>MGSSHHHHHHSQDPAGPIVELDAQGNEIYYRTLSEQHLEILRNNFEVPPTSETFISPLQSYSQEYDGKLVRLTASPGTMNELSKIGVTANSGTGLLLPDLPPARKGWKQNNALFKLEALKKPTIN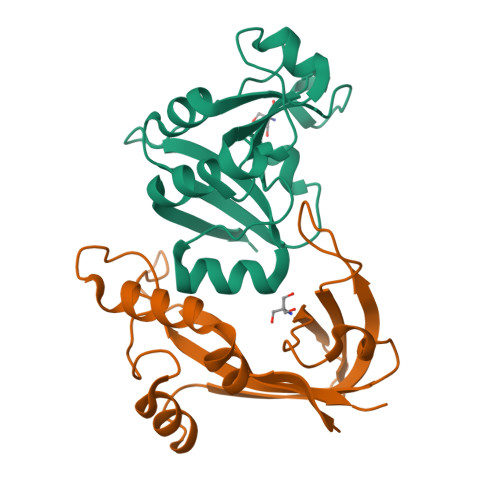EGGGVINTGLGDGKALEIFNKNLIDFEVID[6x];>[6x]MKTIYNFKQRIKEDPEYIRKAHELTLNTTKPKAGLKGTYGLLGSKEWWDNLENGSIPQKEISGTIKKVYLTGQDNTEDFNTIDIETENKTLCTEGTYTNKNTDRKHYEAGKKITIKYAFDPLKKPKPNGDIDYSKIVVEILISE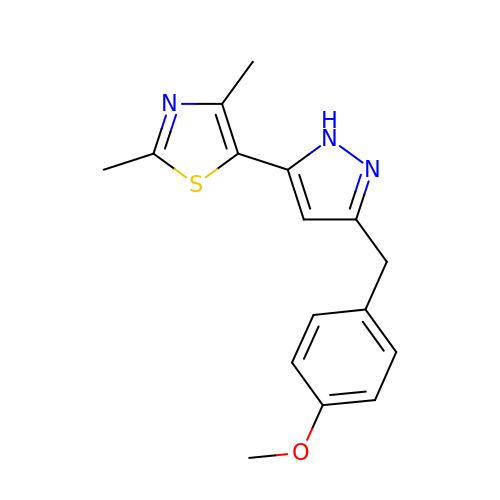5-{3-[(4-methoxyphenyl)methyl]-1H-pyrazol-5-yl}-2,4-dimethyl-1,3-thiazole | C16 H17 N3 O S | SAOOKSMYZRFYPC-UHFFFAOYSA-N> AGQGDGSVIELGEQTVVATAQEETKQAPGVSIITAEDIAKRPPSNDLSQIIRTMPGVNLTGNSSSGQRGNNRQIDIRGMGPENTLILVDGKPVSSRNSVRYGWRGERDSRGDTNWVPADQVERIEVIRGPAAARYGNGAAGGVVNIITKQAGAETHGNLSVYSNFPQHKAEGASERMSFGLNGPLTENLSYRVYGNIAKTDSDDWDINAGHESNRTGKQAGTLPAGREGVRNKDIDGLLSWRLTPEQTLEFEAGFSRQGNIYTGDTQNTNSNNYVKQMLGHETNRMYRETYSVTHRGEW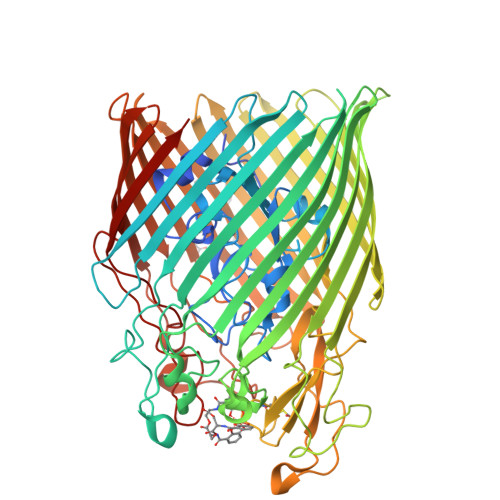DFGSSLAYLQYEKTRNSRINEGLAGGTEGIFDPNNAGFYTATLRDLTAHGEVNLPLHLGYEQTLTLGSEWTEQKLDDPSSNTQNTEEGGSIPGLAGKNRSSSSSARIFSLFAEDNIELMPGTMLTPGLRWDHHDIVGDNWSPSLNLSHALTERVTLKAGIARAYKAPNLYQLNPDYLLYSRGQGCYGQSTSCYLRGNDGLKAETSVNKELGIEYSHDGLVAGLTYFRNDYKNKIESGLSPVDHASGGKGDYANAAIYQWENVPKAVVEGLEGTLTLPLADGLKWSNNLTYMLQSKNKETGDVLSVTPRYTLNSMLDWQATDDLSLQATVTWYGKQKPKKYDYHGDRVTGSANDQLSPYAIAGLGGTYRLSKNLSLGAGVDNLFDKRLFRAGNAQGVVGIDGAGAATYNEPGRTFYTSLTASF Containing a tandem array of 2–30 repeats, pentatricopeptide repeat (PPR) proteins constitute one of the largest protein families in land plants. Each PPR repeat aligns to a single nucleotide of the RNA target in modular patterns, making these proteins suitable for the development of exciting new biotechnologies. Within each repeat, the combinations of two amino acids, known as the PPR code at two key positions (the 5th and the 35th) confer RNA specificity. A typical RNA-bound dPPR protein adopts a right-handed superhelical spiral structure, with its target ssRNA molecule sitting in the interior cavity and interacting with corresponding PPR repeats in a modular fashion.

To verify the RNA selectivity, the dPPR proteins dPPR-U8N2 (in which N indicates any nucleotide) comprising 10 dPPR repeats with different 5th and 6th repeats with different PPR codes were constructed and purified to homogeneity. After numerous unsuccessful trials, we finally succeeded in crystallizing each dPPR-U8N2 in complex with its respective target ssRNA (5′-UUUUNNUUUU-3′), in space group P212121. Because the four structures exhibited almost identical features except for the RNA base binding details of repeats 5 and 6, we focused on describing the structure of RNA-bound dPPR-U8C2. In the complex structure, dPPR-U8C2 has 10 dPPR repeats (residues 174–523), which are capped by NTD and CTD helices. Each repeat in dPPR-U8C2 contains 35 amino acids, forming a hairpin of α-helices that both contain four helical turns followed by a five-residue loop. The whole-protein molecule has an overall appearance of a solenoid with a polar axis of 75 Å and a diameter of  50 Å. Although it has a similar diameter to RNA-free cPPR-polyC and synthPPR3.5, RNA-bound dPPR-U8C2 exhibits a more compact conformation with a helical period length of ∼70 Å, which is shorter than that of cPPR proteins (∼90 Å). We observed that water molecules between bases and PPR repeats mediate hydrogen bonds between the polar residues and the bases in the cases of uracil and cytosine recognition. Each water molecule between the base and corresponding PPR repeat forms two hydrogen bonds: one with the N3 atom of the pyrimidine and one with the carboxyl group of Asp35 or the hydroxyl group of Ser35. The N3 atom of uracil is a hydrogen bond donor, whereas the N3 atom of cytosine is a hydrogen bond acceptor.

> ALLDETPLPPGSRLDVRAYTTVLHALSRAGRYERALELFAELRRQGVAPTVVTYNTLIDGLCKAGKLDEALKLFEEMVEKGIKPDVVTYNTLIDGLCKAGKLDEALKLFEEMVEKGIKPDVVTYNTLIDGLCKAGKLDEALKLFEEMVEKGIKPDVVTYNTLIDGLCKAGKLDEALKLFEEMVEKGIKPDVVTYNTLIDGLCKAGKLDEALKLFEEMVEKGIKPSVVTYNTLIDGLCKAGKLDEALKLFEEMVEKGIKPSVVTYNTLIDGLCKAGKLDEALKLFEEMVEKGIKPDVVTYNTLIDGLCKAGKLDEALKLFEEMVEKGIKPDVVTYNTLIDGLCKAGKLDEALKLFEEMVEKGIKPDVVTYNTLIDGLCKAGKLDEALKLFEEMVEKGIKPDELTYRRVVESYCRAKRFEEARGFLSEVSETDLDFDKKALEAYIEDAQFGRLEHHHHHHHH>XSDIAFLIDGSGSIIPHDFRRMKEFVSTVMEQLKKSKTLFSLMQYSEEFRIHFTFKEFQNNPNPRSLVKPITQL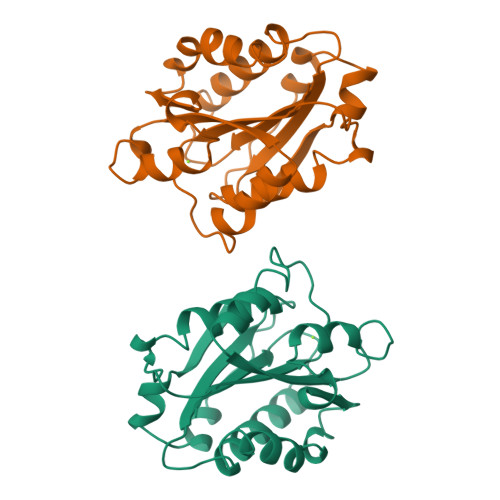LGRTHTATGIRKVVRELFNITNGARKNAFKILVVITDGEKFGDPLGYEDVIPEADREGVIRYVIGVGDAFRSEKSRQELNTIASKPPRDHVFQVNNFEALKTIQNQLREKIFAIEG[2x]>[2x]MRMRHKPWWDDFLAENADIAISNPADYKGKWNTVFGNDNPIHIEVGTGKGQFISGMAKQNPDINYIGIELFKSVIVTAVQKVKDSEAQNVKLLNIDADTLTDVFEPG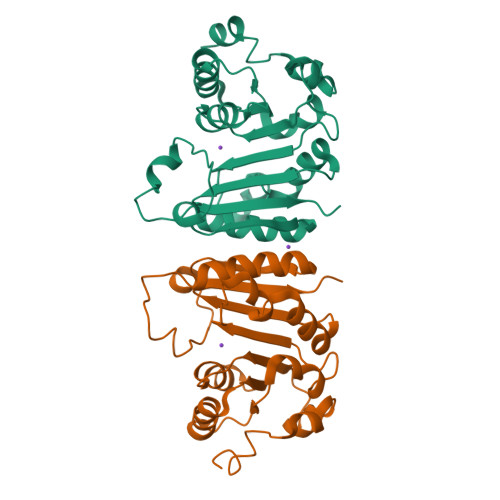EVKRVYLNFSDPWPKKRHEKRRLTYSHFLKKYEEVMGKGGSIHFKTDNRGLFEYSLKSFSEYGLLLTYVSLDLHNSNLEGNIMTEYEEKFSALGQPIYRAEVEWRT> MGSDKIHHHHHHMILVYSTFPNEEKALEIGRKLLEKRLIACFNAFEIRSGYWWKGEIVQDKEWAAIFKTTEEKEKELYEELRKLHPYETPA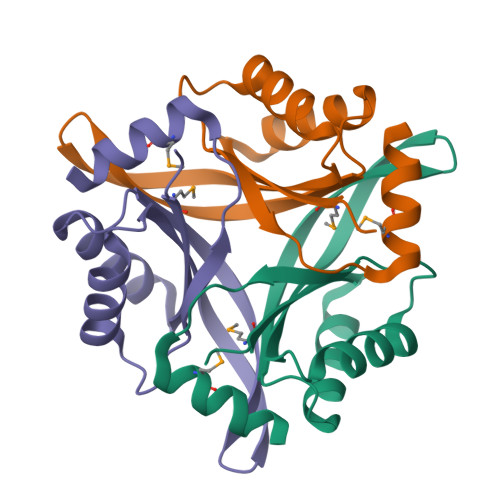IFTLKVENVLTEYMNWLRESVL>[2x]PFTYSIEATRNLATTERCIQDIRNAPVRNRSTQFQLAQQNMLAYTFGEVIPGFASAGINGMDYRDVIGRPVENAVTEGTHFFRDDFRVDSNAKAKVAGDIFEIVSS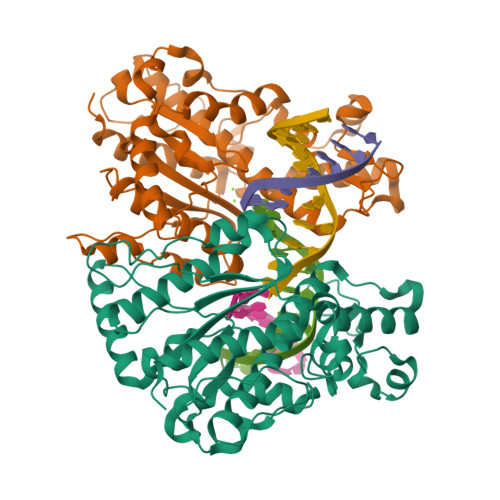AVMWNCAARWNSLMVGEGWRSQPRYSRPTLSPSPRRQVAVLNLPRSFDWVSLLVPESQEVIEEFRAGLRKDGLGLPTSTPDLAVVVLPEEFQNDEMWREEIAGLTRPNQILLSGAYQRLQGRVQPGEISLAVAFKRSLRSDRLYQPLYEANVMQLLLEGKLGAPKVEFEVHTLAPEGTNAFVTYEAASLYGLAEGRSAVHRAIRELYVPPTAADLARRFFAFLNERMELVNG>[2x]TADELVFFVNGKKVVEKNADPETTLLAYLRRKLGLRGTKLGCGEGGCGACTVMLSKYDRLQDKIIHFSANACLAPICTLHHVAVTTVEGIGSTKTRLHPVQERIAKSHGSQCGFCTPGIVMSMYTLLRNQPEPTVEEIEDAFQGNLCRCTGYRPILQGFRTFAK;>PKQLRFEGERVTWIQASTLKELLDLKAQHPEAKLVVGNTEIGIEMKFKNQLFPMIICPAWIPELNAVEHGPEGISFGAACALSSVEKTLLEAVAKLPTQKTEVFRGVLEQLRWFAGKQVKSVASLGGNIITASPISDLNPVFMASGTKLTIVSRGTRRTVPMDHTFFPSYRKTLLGPEEILLSIEIPYSREDEFFSAFKQASRREDDIAKVTCGMRVLFQPGSMQVKELALCYGGMADRTISALKTTQKQLSKFWNEKLLQDVCAGLAEELSLSPDAPGGMIEFRRTLTLSFFFKFYLTVLKKLG[2x];>[2x]DTVGRPLPHLAAAMQASGEAVYCDDIPRYENELFLRLVTSTRAHAKIKSIDVSEAQKVPGFVCFLSADDIPGSNETGLFNDETVFAKDTVTCVGHIIGAVVADTPEHAERAAHVVKVTYEDLPAIITIEDAIKNNSFYGSELKIEKG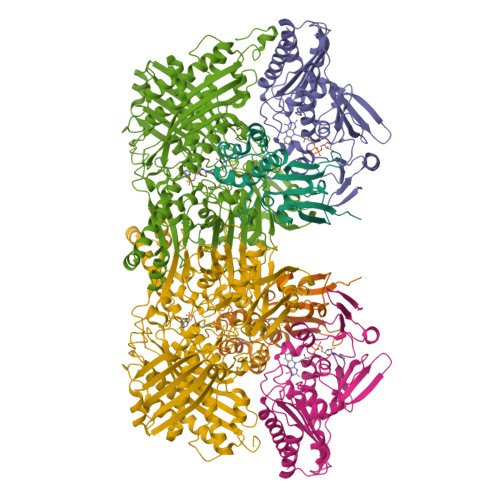DLKKGFSEADNVVSGELYIGGQDHFYLETHCTIAIPKGEEGEMELFVSTQNAMKTQSFVAKMLGVPVNRILVRVKRMGGGFGGKETRSTLVSVAVALAAYKTGHPVRCMLDRNEDMLITGGRHPFLARYKVGFMKTGTIVALEVDHYSNAGNSRDLSHSIMERALFHMDNCYKIPNIRGTGRLCKTNLSSNTAFRGFGGPQALFIAENWMSEVAVTCGLPAEEVRWKNMYKEGDLTHFNQRLEGFSVPRCWDECLKSSQYYARKSEVDKFNKENCWKKRGLCIIPTKFGISFTVPFLNQAGALIHVYTDGSVLVSHGGTEMGQGLHTKMVQVASKALKIPISKIYISETSTNTVPNSSPTAASVSTDIYGQAVYEACQTILKRLEPFKKKNPDGSWEDWVMAAYQDRVSLSTTGFYRTPNLGYSFETNSGNAFHYFTYGVACSEVEIDCLTGDHKNLRTDIVMDVGSSLNPAIDIGQVEGAFVQGLGLFTLEELHYSPEGSLHTRGPSTYKIPAFGSIPTEFRVSLLRDCPNKKAIYASKAVGEPPLFLGASVFFAIKDAIRAARAQHTNNNTKELFRLDSPATPEKIRNACVDKFTTLCVTGAPGNC>[2x]MVNGKVALVTGAAQGIGRAFAEALLLKGAKVALVDWNLEAGVQCKAALDEQFEPQKTLFIQCDVADQQQLRDTFRKVVDHFGRLDILVNNAGVNNEKNWEKTLQINLVSVISGTYLGLDYMSKQNGGEGGIIINMSSLAGLMPVAQQPVYCASKHGIVGFTRSAALAANLMNSGVRLNAICPGFVNTAILESIEKEENMGQYIEYKDHIKDMIKYYGILDPPLIANGLITLIEDDALNGAIMKITTSKGIHFQDY

The enzyme 15-prostaglandin dehydrogenase (15-PGDH) is a key negative regulator of tissue stem cell activity in proliferation and in the repair of tissue injury, whose negative regulation of tissue regeneration is conserved across multiple organs. 15-PGDH acts via its NAD+-dependent enzymatic activity of oxidizing and degrading prostaglandin E2 (PGE2), and related eicosanoids, which provide key trophic support for stem cells in multiple tissues. Specifically, 15-PGDH catalyzes the rate-limiting step to initiate PGE2 degradation by oxidizing the 15-hydroxyl moiety of PGE2 to a 15-keto group, thereby inactivating PGE2 from being able to bind to its receptors. 15-PGDH assembled as a homodimer, which is the proposed physiological form of the enzyme.

To examine the generality of the molecular interactions that govern 15-PGDH inhibition, we expanded our investigation to include a newer generation of 15-PGDH inhibitors, SW22274613 that represents an entirely different chemical scaffold. SW222746, has a similar IC50 as (+)-SW209415, but is based on a quinoxaline scaffold that is chemically distinct from the thienopyridine-based structure of (+)-SW209415. We used cryo-EM to define the molecular interactions of SW222746-bound to 15-PGDH, which were interpreted from the structure determined with an average resolution of 2.9 Å. Strikingly, SW222746 occupies a nearly identical pocket as that of (+)-SW209415, while using different chemical groups to maintain critical interactions with key 15-PGDH residues. Specifically, as was the case with (+)-SW209415, SW222746 is fully encapsulated in the drug binding pocket with the α10-α12 lid of 15-PGDH closed around it. Similar to (+)-SW209415, the closing of the lid again appears to be orchestrated through π-stacking interactions coordinated through F185 and Y217 of 15-PGDH with the quinoxaline and quinoline-2(1H)- moieties, respectively, of SW222746. The amide carbonyl group of SW222746 replaces the (+)-SW209415 sulfoxide and maintains the specific recognition of the catalytic core of the enzyme through, again, a hydrogen bonding network formed with the critical S138 and Y151 residues. The piperidine moiety of SW222746 replaces the butyl chain of (+)-SW209415 to maintain hydrophobic interactions as well. For example, the thienopyridine of (+)-SW209415 reaches into the catalytic pocket to form a hydrogen bond (amine group at position 3) with Q148 of 15-PGDH, whereas SW222746 does not form any interactions with Q148. Additionally, the elongated quinoxaline and quinoline-2(1H)-one moiety of SW222746 form interactions with T246 within the β7 strand of 15-PGDH that is not observed for (+)-SW209415 binding to the protein, and interactions with Y217 are stronger for SW222746 than for (+)-SW209415 (Fig. 1e vs 4e).> RKAYPECGENEWLDDCGTQKPCEAKCNEEPPEEEDPIC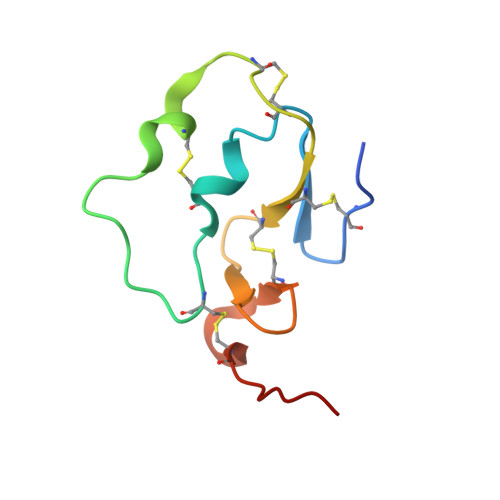RSRGCLLPPACVCKDGFYRDTVIGDCVREEECDQHEIIHV>[2x]ALPDLKIEKLEEGVFVHTSFEEVNGWGVVTKHGLVVLVNTDAYLIDTPFTATDTEKLVNWFVERGYEIKGTISSHFHSDSTGGIEWLNSQSIPTYASELTNELLKKSGKVQAKYSFSEVSYWLVKNKIEVFYPGPGHTQDNLVVWLPESKILFGGCFIKPHGLGNLGDANLEAWPKSAKILMSKYGKAKLVVSSHSEKGDASLMKRTWEQALKGLKESKKTSSPSN

IMP-13, a member of subgroup 2, sharing 92.3% amino acid sequence similarity with IMP-2 and 82.5% with IMP-1 (Fig. SI2), was first identified in the Gram-negative pathogen Pseudomonas aeruginosa from clinical samples in Italy and is a common cause of carbapenem resistance, often involved in large outbreaks. Imipenemases represent one of the major groups of class B1 metallo-β-lactamases found in Gram-negative pathogens, and these enzymes can hydrolyze all bicyclic β-lactam antibiotics. The overall protein architecture of the IMP-13 apo structure is consistent with that of the previously published metallo-β-lactamase fold, consisting of a global αβ/βα topology with a shallow active-site cleft at the border of the two β-sheets. The structural information and dynamics presented here reveal important information about the mechanism of antibiotic binding, as well as a significant role for the active-site-covering loop (L1), indicating that the plasticity of the active-site region is important for the broad substrate recognition spectrum of these enzymes.

In complex with each of the hydrolyzed carbapenems, this loop forms a tightly locked, tunnel-like structure around the hydrolyzed antibiotic, with several hydrophobic interactions appearing to stabilize this state. The sulfur atom present in the linker region (S-10) of all carbapenems creates strong π-sulfur interactions with the aromatic ring of Trp28 (as well as interacting with the backbone of Asn167), thereby contributing to the position of the core scaffold of all presented carbapenem substrates. The pyrrolidine ring of meropenem, doripenem, and ertapenem is suitably located to form aromatic, π-alkyl interactions with His197 and is further stabilized by the hydrophobic environment created by Val25 and Val31. The terminal nitromethyl group of meropenem is stabilized by direct as well as water-mediated interactions with the backbone of His163 and Gly164 and π-alkyl interactions with Trp28. In the X-ray structures, the interaction of bound ertapenem and meropenem with the Trp28 side chain occurs via the sulfur adjacent to the β-lactam ring and, additionally, via the methyl group on the pyrroline ring. Further description focuses on chain B of the doripenem-, ertapenem-, and imipenem-bound structures and chain A of the meropenem-bound structure, where crystal packing is not seen to affect ligand placement. The lower root mean squared fluctuations (RMSFs) for heavy atoms of L1 residues in the simulated doripenem-, ertapenem-, and meropenem-bound complex structures than for those of the apoclosed structure indicate that L1 is more rigid in the closed conformation when these ligands are bound, while in the apo protein, L1 can move with a higher degree of freedom. Nevertheless, it is clear from the MD simulations that differences in antibiotic structure affect the restriction of the L1 loop, with the doripenem, ertapenem, and meropenem complexes showing the greatest restriction in L1 loop mobility.AMPylation (adenylylation) is an evolutionarily conserved PTM characterized by the covalent addition of adenosine monophosphate (AMP) to the hydroxyl side chains of amino acids in protein substrates. We developed a strategy to enrich for AMPylated proteins using the histidine triad nucleotide-binding protein, hinT. Although its physiological substrates are still unknown, in vitro characterization of hinT revealed high-affinity purine nucleotide binding and phosphoramidase activity. To investigate the structural mechanisms of AMPylated protein binding to hinTHN, we used AMPylated GlnA (GlnA-AMP) as a model substrate.

We solve the cryo-EM structure of an AMPylated protein bound to the nucleotide binding pocket of hinT to provide structural insights into the mechanism of substrate recognition and specificity. Focused refinement of hinTHN depicted the flexible loops of GlnA-AMP extending into the binding pocket of hinTHN. The hinTHN dimer binds two GlnA molecules, with each hinTHN subunit interacting slightly differently. Some interactions are similar between the subunits, such as Ile32 interacting with the adenine group. In addition, Met113 extends into the binding pocket of the neighboring hinT, coming into close proximity with the AMPylated amino acid, Tyr398, of GlnA-AMP. His103 of both subunits are next to the phosphate group of AMP, likely making polar contacts with the oxygens of the phosphate group. The structure of hinT bound to AMPylated GlnA depicts the AMP moiety of Tyr-AMP bound in the nucleotide binding pocket with unique interactions that precisely coordinate the phosphate and purine ring. Notably, Glu96, which is in close proximity to the phosphate moiety in E. coli hinT, is not conserved in human and T. marianensis homologs of hinT. However, the negatively charged glutamate may induce repulsion, contributing to the reduced affinity for AMPylated proteins observed with E. coli hinT. The structure of AMPylated GlnA bound to hinT provides a platform for protein engineering to optimize the binding interface to alter specificity and sensitivity for AMPylated proteins.

>[2x]SEFELMSAEHVLTMLNEHEVKFVDLRFTDTKGKEQHVTIPAHQVNAEFFEEGKMFDGSSIGGWKGINESDMVLMPDASTAVIDPFFADSTLIIRCDILEPGTLQGYDRDPRSIAKRAEDYLRSTGIADTVLFGPEPEFFLFDDIRFGSSISGSHVAIDDIEGAWNSSTQYEGGNKGHRPAVKGGYFPVPPVDSAQDIRSEMCLVMEQMGLVVEAHHHEVATAGQNEVATRFNTMTKKADEIQIYKYVVHNVAHRFGKTATFMPKPMFGDNGSGMHCHMSLSKNGVNLFAGDKYAGLSEQALYYIGGVIKHAKAINALANPTTNSYKRLVPGYEAPVMLAYSARNRSASIRIPVVSSPKARRIEVRFPDPAANPYLCFAALLMAGLDGIKNKIHPGEAMDKNLYDLPPEEAKEIPQVAGSLEEALNELDLDREFLKAGGVFTDEAIDAYIALRREEDDRVRMTPHPVEFELYYSV;>[2x]GAMGSMAEETIFSKIIRREIPSDIVYQDDLVTAFRDISPQAPTHILIIPNILIPTVNDVSAEHEQALGRMITVAAKIAEQEGIAEDGYRLIMNTNRHGGQEVYHINMHLLGGRPLGPMLAHKGL> MGSDRSCVLSVFQTILKLVIFVAIFGAAISSRLFAVIKFESIIHEFDPWFNYRATKYLVNNSFYKFLNWFDDRTWYPLGRVTGGTLYPGLMTTSAFIWHALRNWLGLPIDIRNVCVLFAPLFSGVTAWATYEFTKEIKDASAGLLAAGFIAIVPGYISRSVAGSYDNEAIAITLLMVTFMFWIKAQKTGSIMHATCAALFYFYMVSAWGGYVFITNLIPLHVFLLILMGRYSSKLYSAYTTWYAIGTVASMQIPFVGFLPIRSNDHMAALGVFGLIQIVAFGDFVKGQISTAKFKVIMMVSLFLILVLGVVGLSALTYMGLIAPWTGRFYSLWDTNYAKIHIPIIASVSEHQPVSWPAFFFDTHFLIWLFPAGVFLLFLDLKDEHVFVIAYSVLCSYFAGVMVRLMLTLTPVICVSAAVALSKIFDIYLDFKTSDRKYAIKPAALLAKLIVSGSFIFYLYLFVFHSTWVTRTAYSSPSVVLPSQTPDGKLALIDDFREAYYWLRMNSDEDSKVAAWWDYGYQIGGMADRTTLVDNNTWNNTHIAIVGKAMASPEEKSYEILKEHDVDYVLVIFGGLIGFGGDDINKFLWMIRISEGIWPEEIKERDFYTAEGEYRVDARASETMRNSLLYKMSYKDFPQLFNGGQATDRVRQQMITPLDVPPLDYFDEVFTSENWMVRIYQLKKDDAQGRTLRDVGELTRSSTKTRRSIKRPELGLRV;> MISDEQLNSLAITFGIVMMTLIVIYHAVDSTMSPKNRTLQVDGGSGGSLEVLFQGPTETSQVAPA;> MTYEQLYKEFHSSKSFQPFIHLDTQPKFAICGLIVTLAVLSSALFAVGSKSSYIKKLFFYTILSVIGSLFAGLTTVFASNSFGVYV;> MAKAPKANTPKVTSTSSAVLTDFQETFKTSKRAYFAQIEKYPKLKLIDTFCFFLVLLGVIQCTFIILIRDNFPFNAFLAGFIICVGQFVLLMSLRLQLCNSFPGISKNRAFAEFIVASLILHFVCLHFIN;> MRQVWFSWIVGLFLCFFNVSSAAQYEPPATWENVDYKRTIDVSNAYISETIEITIKNIASEPATEYFTAFESGIFSKVSFFSAYFTNEATFLNSQLLANSTTAPGDDGESEIRYGIIQFPNAISPQEEVSLVIKSFYNTVGIPYPEHVGMSEEQHLLWETNRLPLSAYDTKKASFTLIGSSSFEEYHPPNDESLLGKANGNSFEFGPWEDIPRFSSNETLAIVYSHNAPLNQVVNLRRDIWLSHWASTIQFEEYYELTNKAAKLSKGFSRLELMKQIQTQNMRQTHFVTVLDMLLPEGATDHYFTDLVGLVSTSHAERDHFFIRPRFPIFGGWNYNFTVGWTNKLSDFLHVSSGSDEKFVASIPILNGPPDTVYDNVELSVFLPEGAEIFDIDSPVPFTNVSIETQKSYFDLNKGHVKLTFSYRNLISQVANGQVLIKYDYPKSSFFKKPLSIACYIFTALMGVFVLKTLNMNVTN;> MQFFKTLAALVSCISFVLAYVAQDVHVSFPSTAGKSRVMIGKVEPRIGIDETVPTTITVEDPNEVIQVNFAIESTNKPFQNTLLIGLPNKNLEMAFEPEIKDNGKLSMYKYRIDLAKLDAALLQEASRSPEPIKATLILASSTAKPKENLFREILQLNLNFDVDHSDSSLVDKFGIKPEIHHIFHAEPKRVAKPIAVIFVLIIFITILSLIVTWLNSCAAAFNNIPTGVTAVYFLGFIATIVGFEVIFARYYLGTSIFETLFSSLYLGAPGLLTSTKFLRSFG;> MRTDWNFFFCILLQAIFVVGTQTSRTLVLYDQSTEPLEEYSVYLKDLEQRNYKLEYLDINSTSTTVDLYDKEQRLFDNIIVFPTKGGKNLARQIPVKQLIKFFENEGNILCMSSPGAVPNTIRLFLNELGIYPSPKGHVIRDYFSPSSEELVVSSNHLLNKYVYNARKSEDFVFGESSAALLENREQIVPILNAPRTSFTESKGKCNSWTSGSQGFLVVGFQNLNNARLVWIGSSDFLKNKNQDSNQEFAKELLKWTFNEKSVIKSVHAVHSHADGTSYDEEPYKIKDKVIYSVGFSEWNGEEWLPHIADDIQFELRQVDPYYRLTLSPSGNDSETQYYTTGEFILPDRHGVFTFLTDYRKIGLSFTTDKDVKAIRHLANDEYPRSWEISNSWVYISAICGVIVAWIFFVVSFVTTSSVGKKLETFKKTN;> MNWLFLVSLVFFCGVSTHPALAMSSNRLLKLANKSPKKIIPLKDSSFENILAPPHENAYIVALFTATAPEIGCSLCLELESEYDTIVASWFDDHPDAKSSNSDTSIFFTKVNLEDPSKTIPKAFQFFQLNNVPRLFIFKPNSPSILDHSVISISTDTGSERMKQIIQAIKQFSQVNDFSLHLPMDWTPIITSTIITFITVLLFKKQSKLMFSIISSRIIWATLSTFFIICMISAYMFNQIRNTQLAGVGPKGEVMYFLPNEFQHQFAIETQVMVLIYGTLAALVVVLVKGIQFLRSHLYPETKKAYFIDAILASFCALFIYVFFAALTTVFTIKSPAYPFPLLRLSAPFK;> YANATSA

Oligosaccharyltransferase (OST) is the central enzyme of N-linked protein glycosylation. It catalyzes the transfer of a pre-assembled glycan, GlcNAc2Man9Glc3, from a dolichyl-pyrophosphate donor to acceptor sites in secretory proteins in the lumen of the endoplasmic reticulum. In higher metazoans and fungi, OST is a multimeric complex composed of eight subunits spatially arranged in three subcomplexes that are formed during OST assembly. Subcomplex I contains OST1 and OST5; subcomplex II contains OST3 (or OST6), STT3, and OST4; and subcomplex III contains OST2, WBP1, and SWP1.

To distinguish the effects of bound LLO and peptide on the 3D conformation of OST, we determined a separate structure of yeast OST bound to the reactive peptide TAMRA-YANATS-NH2 but in the absence of LLO. A comparison with the ternary complex structure (containing Dab peptide) revealed indistinguishable peptide pose and conformation, suggesting that the Dab residue used for the ternary complex structure had not altered the conformation of OST. Conversely, binding of an acceptor peptide alone to the apo-state engages the C-terminal half of EL5 (EL5-C) only, and does not involve TM9. This still allows the subsequent binding of LLO that now engages the N-terminal half of EL5 (EL5-N) and TM9. Peptide-primed: if the next glycosylation sequon is closely spaced, it can bind to OST, leading to engagement of the C-terminal half of EL5 (EL5-C). We speculate that this is important for the efficient glycosylation of closely spaced sequons, where there is an increase in the local sequon concentration, and a peptide-primed OST is more likely to be formed.NoVs recognize specific glycan ligands as host attachment factors or receptors for infection. NoVs interact with HBGAs or other glycans through their capsid protrusions that are built by the dimeric protruding (P) domain of NoV capsid protein (VP1). Genogroup II (GII) noroviruses consist of human noroviruses (huNoVs) that generally bind histo-blood group antigens (HBGAs) as host factors and three porcine norovirus (porNoV) genotypes (GII.11/18/19) that form a genetic lineage lacking HBGA-binding ability. In this study, we solved the P protein crystal structures of a GII.11 porNoV (VA34) that was isolated from pig caecum contents in 1997 in Japan and a close-related GII.3 huNoV (TV24) that was isolated in 1977 in the USA, representing one of the earliest huNoV isolates, focusing on their HBSs compared with the previously known ones.

In contrast, the porNoV VA34 P protein did not bind these saliva samples (OD < 0.1) and it did not bind the oligosaccharides representing A, B, and H antigens either (OD < 0.1). Although 10 oligosaccharides representing various HBGAs and a ganglioside were used to co-crystallize with the VA34 P proteins individually, no extra electron density was seen other than the native P protein, consistent with the negative results of HBGA binding assay and glycan array screening. However, the sequence compositions and the structure of the VA34 site corresponding to the HBSs of the TV24 and other GII huNoVs appeared to be conserved (Figures 4 and 7(A and B)), indicating that this site of VA34 is under functional selection over time during evolution. On the other hand, the V451 mutation in the VA34 P protein loses the conserved Van der Waals interaction to the α-Fuc of the HBGAs. Thus, the two mutations damage the structure and function of the HBS and explain the lack of HBGA binding ability of GII.11 porNoV VA34. The primary variations in both sequences and structures between the two P proteins are at the surface loops between β-strands, mainly in the P2 subdomains that form the top surface of the viral protrusions, most likely contributing to the differences in their antigenicity and HBSs. VA34 P protein represents the first solved P protein structure of a GII porNoV.

>[2x]SKTKPFSLPSLTLDELSNSRFPAPIVQLYTNPHDNLVVQPQNGRCTIDGLLQGTTQLVSCNVCSFRGTLGDGQPASHSEEEIMPMAFNIQREIMLENLDGSPYDPTDDIPAVLGSPDFQGVVFGILSQRNTDGQTRAHEAKVDTRLARFAPKLGFVVATVENTDFHANQPCRFTPVGLGGDNNRDFNQWGLPAYGGALTNNTNLAPPVMPVYPGEQLLFFRSQLPSSGGVVGGWLDCLLPQEWVQHFFQESATSQSDVALVRYINPTTGRVLFEAKLHKQGFLTVAASGSYPLVVPADGYFRFESWVNQFYTLAPMGNGSG> MAGVETAVRQIELK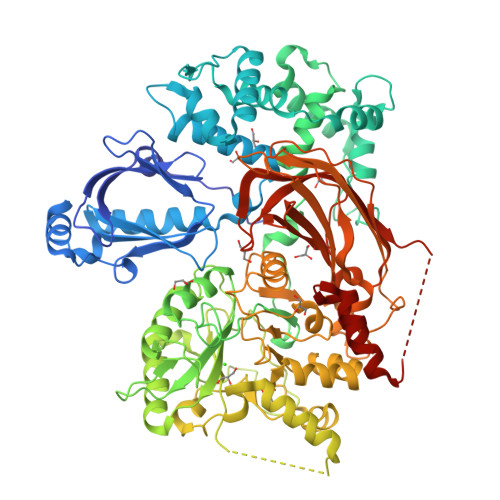WPKVPEQLIKGDKFLKWEEGSSGFIEILLRVDPKGYFLYWKIEGKEDTQLLDLAYVRDIRCAKYAKPPKDKKIKEAGTNFGSSNIPLQDKCVTICHGYNYIDLEWTHLVAENSSVAKKWSEEVFSYAYNLLSLNKNQLGEWEKLYFRLTTVEMEKNKIPVKAIQKCLSKDKDDRARISKALEKIGWPSGKNDAIDLKAFDFDTFFKFYLALLERSEIEGIFKELSKNKGNITTVMFRDFLNDMQRHPSLHKTLFPLYTDAQCEALINDYESAVNKKGKKKGQLTKEGLLYFLMCEENNLTPMHRLDLGANMKLTLAAYYINSSHNTYLTGHQLTGKSSVEIYRQVLLTGCRCLELDCWDGKDGEPIITHGFTMCTEVLFKDVVYAIAESAFKVSDYPVILSFENHCSVAQQKLLAQYCNEAFGELLLDKPIDGHPLKPGVPLPTPYDLRKKILIKNKKMHKGTGDDEELAGLTDEEKKKIEKEKKDAGTAAKEAEAAEEMSALVNYIQPVHFTTFEQAQKKDRHYEMSSMVETQALNKLKDNPEDFVDYNKKQITRIYPKGTRVDSSNYVPQIYWNAGCQLVALNFQCFDIAMCVNLGVFEYNGCSGYLLKPEFMRKLDKRFDPFTESTVDGVVAGTIEIKIISAQFLSDKQISSYVEVEMYGLPTDTVRKKFKTKIIENNGMDPYYDEKVFVFKKVVLPDLAVVRIIVSEENGKFIGHRVMPLDGIKPGYRHVPLRNESNRPLGLASVFAHIVAKDYVSDAFADFADALLNPIAYQSAQEARAAALCAFEDDPDAALNAAK> MAAALSEQLAELEKRSGGRLGVAVLDTATGRRFGYRGDERFPMCSTFKALLAAAVLARVDQGKENLDRRITYGKEDLVDYSPVTEKHVGDGMTVAELCEAAITYSDNTAANLLLEALGGPAALTAFLRSIGDNVTRLDRWEPELNTAAPGDPRDTTTPAAMAATLRTLLLGDVLS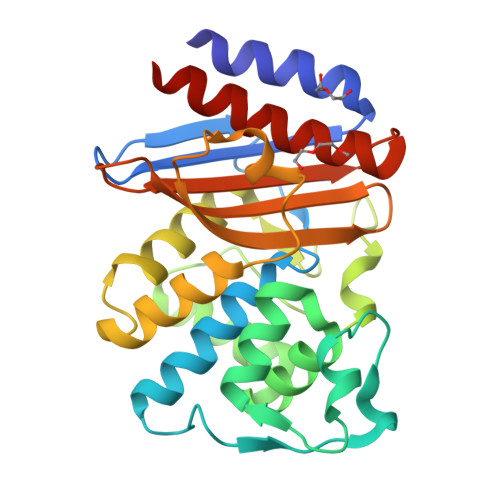PASRQQLVDWLIANKTGDKRLRAGLPADWRVGDKTGTGEHGTTNDIAVIWPPNRAPILVAVYLTESQVDADARDAVIAEVARLVVAAFHHHHHH>[4x]MEMRVLLIAGGVSPEHEVSLLSAEGVLRHIPFPTDLAVIAQDG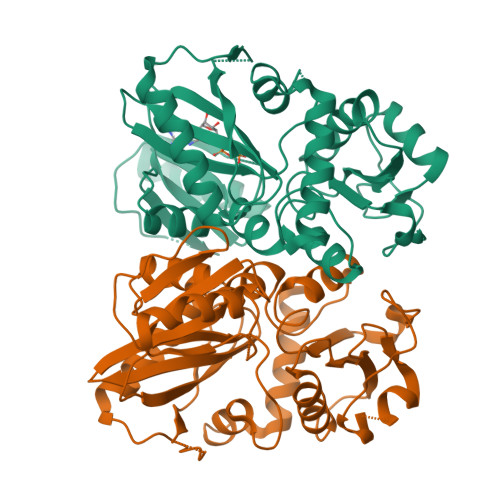RWLLGEKALTALEAKAAPEGEHPFPPPLSWERYDVVFPLLHGRFGEDGTVQGFLELLGKPYVGAGVAASALCMDKDLSKRVLAQAGVPVVPWVAVRKGEPPVVPFDPPFFVKPANTGSSVGISRVERFQDLEAALALAFRYDEKAVVEKALSPVRELEVGVLGNVFGEASPVGEVRYEAPFYDYETKYTPGRAELLIPAPLDPGTQETVQELALKAYKVLGVRGMARVDFFLAEGELYLNELNTIPGFTPTSMYPRLFEAGGVAYPELLRRLVELALTHHHHHH In this context, the highly active, efficient, and selective metal-dependent Formate Dehydrogenases (Fdh) are very appealing systems that enable harnessing millions of years of natural evolution. Additionally, [4Fe–4S] clusters are present to convey electrons to/from the physiological partners. Additionally, the oxygen sensitivity of these enzymes must also be understood as it poses an important obstacle for biotechnological applications. This work presents a combined biochemical, spectroscopic, and structural characterization of Desulfovibrio vulgaris FdhAB (DvFdhAB) when exposed to oxygen in the presence of a substrate (formate or CO2).

A similar approach was employed to gain further insight into the structural changes occurring when the formate-reduced enzyme is exposed to O2, thus rendering it inactivated. Since the formate-reduced enzyme is more sensitive to O2, formate-treated DvFdhAB crystals were first prepared in the anaerobic chamber (<0.1 ppm of O2). Thus, in the current work, the non-activated enzyme (C845–C872 disulfide bond oxidized) was used to slow down the catalytic reaction, aiming at trapping putative intermediates. The formate-reduced DvFdhAB crystals were flash cooled in liquid nitrogen at different time points after exposure to atmospheric O2 (Tables 1 and S1†).

> MTVTRRHFLKLSAGAAVAGAFTGLGLSLAPTVARAELQKLQWAKQTTSICCYCAVGCGLIVHTAKDGQGRAVNVEGDPDHPINEGSLCPKGASIFQLGENDQRGTQPLYRAPFSDTWKPVTWDFALTEIAKRIKKTRDASFTEKNAAGDLVNRTEAIASFGSAAMDNEECWAYGNILRSLGLVYIEHQARIUHSPTVPALAESFGRGAMTNHWNDLANSDCILIMGSNAAENHPIAFKWVLRAKDKGATLIHVDPRFTRTSARCDVYAPIRSGADIPFLGGLIKYILDNKLYFTDYVREYTNASLIVGEKFSFKDGLFSGYDAANKKYDKSMWAFELDANGVPKRDPALKHPRCVINLLKKHYERYNLDKVAAITGTSKEQLQQVYKAYAATGKPDKAGTIMYAMGWTQHSVGVQNIRAMAMIQLLLGNIGVAGGGVNALRGESNVQGSTDQGLLAHIWPGYNPVPNSKAATLELYNAATPQSKDPMSVNWWQNRPKYVASYLKALYPDEEPAAAYDYLPRIDAGRKLTDYFWLNIFEKMDKGEFKGLFAWGMNPACGGANANKNRKAMGKLEWLVNVNLFENETSSFWKGPGMNPAEIGTEVFFLPCCVSIEKEGSVANSGRWMQWRYRGPKPYAETKPDGDIMLDMFKKVRELYAKEGGAYPAPIAKLNIADWEEHNEFSPTKVAKLMNGYFLKDTEVGGKQFKKGQQVPSFAFLTADGSTCSGNWLHAGSFTDAGNLMARRDKTQTPEQARIGLFPNWSFCWPVNRRILYNRASVDKTGKPWNPAKAVIEWKDGKWVGDVVDGGGDPGTKHPFIMQTHGFGALYGPGREEGPFPEHYEPLECPVSKNPFSKQLHNPVAFQIEGEKKAVCDPRYPFIGTTYRVTEHWQTGLMTRRCAWLVEAEPQIFCEISKELAKLRGIGNGDTVKVSSLRGALEAVAIVTERIRPFKIEGVDVHMVGLPWHYGWMVPKNGGDTANLLTPSAGDPNTGIPETKAFMVDVRKVWSHPQFEK;> GKMFFVDLSRCTACRGCQIACKQWKNLPAEETRNTGSHQNPPDLSYVTLKTVRFTEKSRKGPGIDWLFFPEQCRHCVEPPCKGQADVDLEGAVVKDETTGAVLFTELTAKVDGESVRSACPYDIPRIDPVTKRLSKCDMCNDRVQNGLLPACVKTCPTGTMNFGDEQEMLALAEKRLAEVKKTYPGAVLGDPNDVRVVYLFTRDPKDFYEHAVA>[2x]MSVEGLGKDFCGAIIPDNFFPIEKLRNYTQMGLIRDF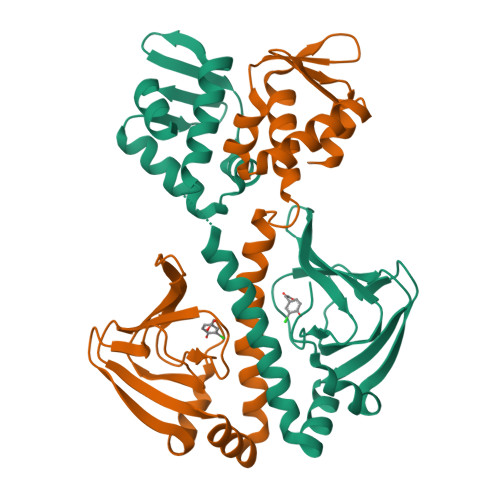AKGSAVIMPGEEITSMIFLVEGKIKLDIIFEDGSEKLLYYAGGNSLIGKLYPTGNNIYATAMEPTRTCWFSEKSLRTVFRTDEDMIFEIFKNYLTKVAYYARQVAEMNTYNPTIRILRLFYELCSSQGKRVGDTYEITMPLSQKSIGEITGVHHVTVSRVLASLKRENILDKKKNKIIVYNLGELKHLSEQTSYYSDPNSSSVDKLAAALDHH>[2x]HHHHHHFNLPPGNYKKPKLLYCSNGGHFLRILPDGTVDGTRDRSDQH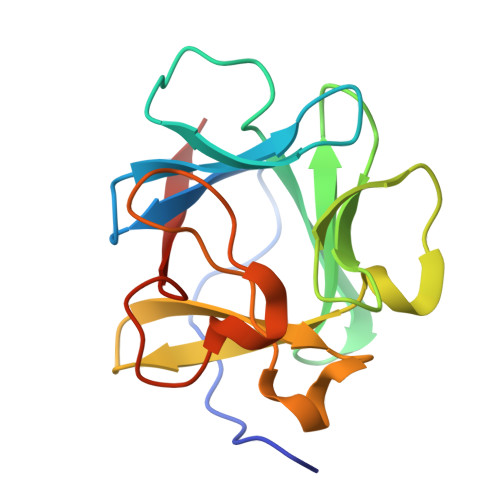IQLQLSAESVGEVYIKSTETGQYLAMDTDGLLYGSQTPNEECLFLERLEENHYNTYISKKHAEKNWFVGLKKNGSCKRGPRTHYGQKAILFLPLPVSSD> ADPDPMKNTCKLLVVADHRFYRYMGRGEESTTTNYLIELIDRVDDIYRNTAWDNAGFKGYGIQIEQIRILKSPQEVKPGEKHYNMAKSYPNEEKDAWDVKMLLEQFSFDIAEEASKVCLAHLFTYQDFDMGTLGLAYVGSPRANSHGGVCPKAYYSPVGKKNIYLNSGLTSTKNYGKTILTKEADLVTTHELGHNFGAEHDPDGLAECAPNEDQGGKYVMYPIAVSGDHENN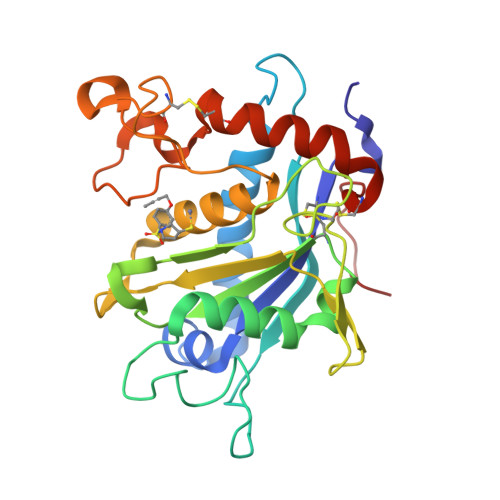KMFSQCSKQSIYKTIESKAQECFQERSNKVIEGR> MRFFLSPPHMGGNELKYIEEVFKSNYIAPLGEFVNRFEQSVKDYSKSENALALNSATAALHLALRVAGVKQDDIVLASSFTFIASVAPICYLKAKPVFI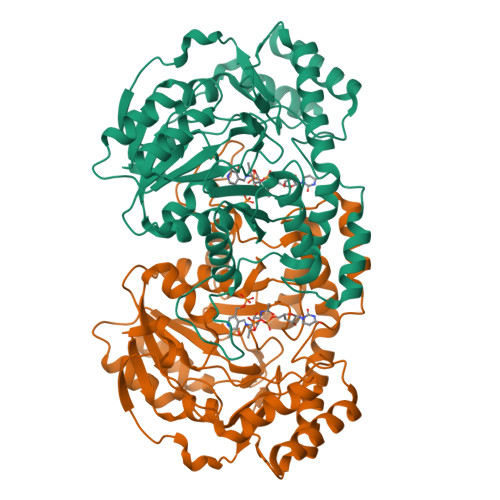DCDETYNIDVDLLKLAIKECEKKPKALILTHLYGNAAKMDEIVEICKENDIVLIEDAAEALGSFYKNKALGTFGEFGVYSYNGNAIITTSGGGMLIGKNKEKIEKARFYSTQARENCLHYEHLDYGYNYRLSNVLGAIGVAQMEVLEQRVLKKREIYEWYKEFLGEYFSFLDELENSRSNRWLSTALINFDKNELNSCQKDINISQKNITLHPKISKLIEDLKNKQIETRPLWKTMHAQEVFKGAKAYLNGNSELFFQKGICLPSGTAMSKDDVYEISKLILKSIKA>SNAALNAAQEKEVRALVRDTLVSNPEILEEAIMALQTKKADEQQAQFRQALASEHDALYNDAASPRIGAKDAKLVLVSFTDYNCPYCKRFDPLLEKITEQYPDVAVIIKPLPFKGESSAKASQAVLSVWKEDPKAF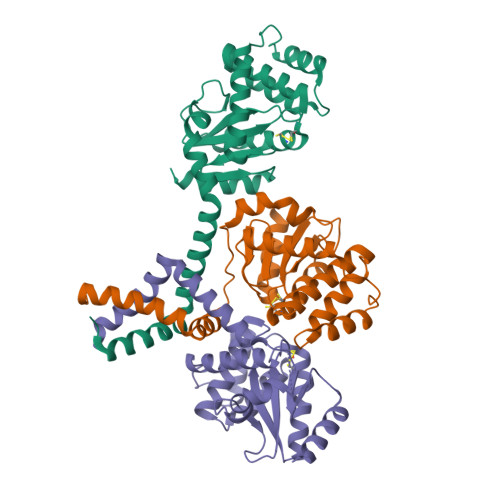LALHQRLMQKKTMLDNASIEDAMKSTNTSKIKLTDDSLKTLQNNLELSRKLGIQGTPATVIGDTILPGAVDYDQLEIIVKEQLAKVKK[6x]> LSSPADSY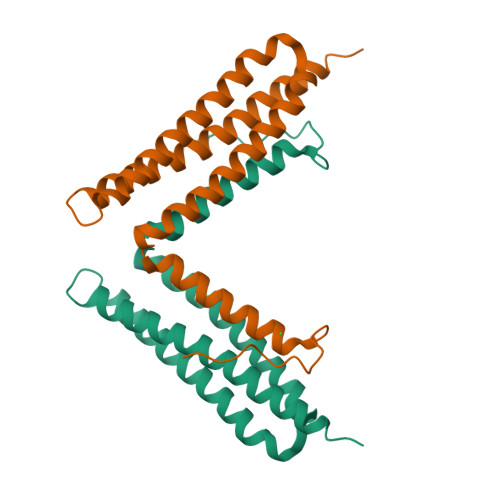NEGVKLQPQEISPPPTANLDRSNDKVYENVTGLVKAVIEMSSKIQPAPPEEYVPMVKEVGLALRTLLATVDETIPLLPASTHREIEMAQKLLNSDLGELINKMKLAQQYVMTSLQQEYKKQMLTAAHALAVDAKNLLDVIDQARLKMLGQTRPH>[2x]GAMEAEHDRSEALLANMLPASIAERLKEPERNIIADKYDEASVLFADIVGFTERASSTAPADLVRFLDRLYSAF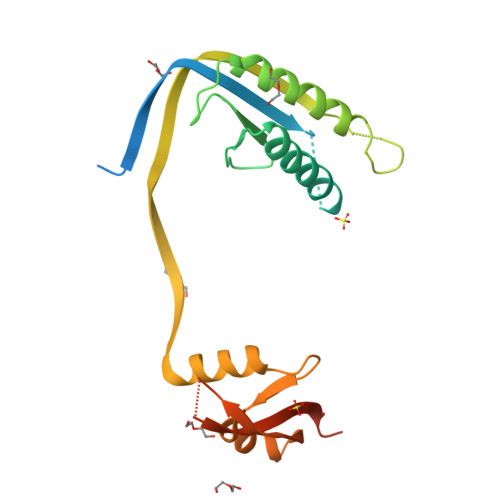DELVDQHGLEKIKVSGDSYMVVSGVPRPRPDHTQALADFALDMTNVAAQLKDPRGNPVPLRVGLATGPVVAGVVGSRRFFYDVWGDAVNVASRMESTDSVGQIQVPDEVYERLKDDFVLRERGHINVKGKGVMRTWYLIGRKVAADPGEVRGAEPRTAGV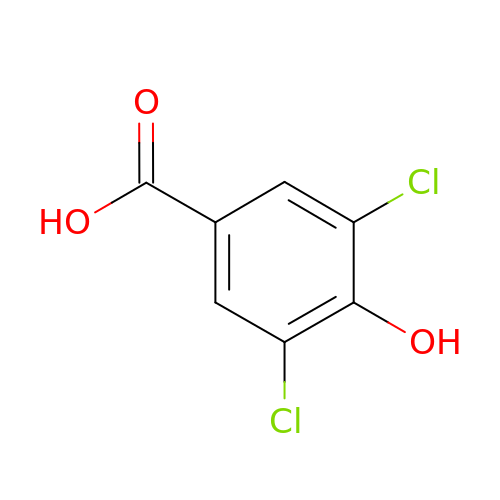3,5-dichloro-4-hydroxybenzoic acid | C7 H4 Cl2 O3 | AULKDLUOQCUNOK-UHFFFAOYSA-N>[5x]MSEKNVSIVVAASVLSSGIGINGQLPWSISEDLKFFSKITNNKCDSNKKNALIMG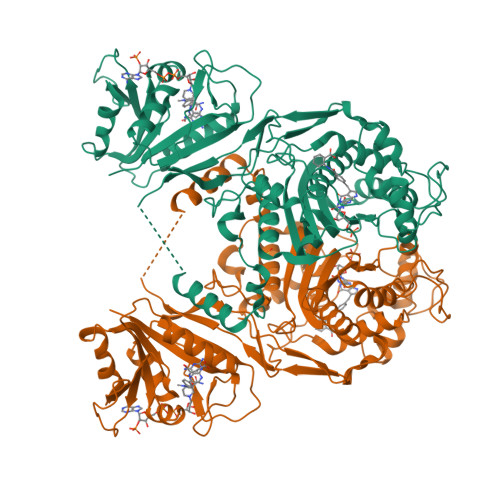RKTWDSIGRRPLKNRIIVVISSSLPQDEADPNVVVFRNLEDSIENLMNDDSIENIFVCGGESIYRDALKDNFVDRIYLTRVALEDIEFDTYFPEIPETFLPVYMSQTFCTKNISYDFMIFEKQEKKTLQNCDPARGQLKSIDDTVDLLGEIFGIRKMGNRHKFPKEEIYNTPSIRFGREHYEFQYLDLLSRVLENGAYRENRTGISTYSIFGQMMRFDMRESFPLLTTKKVAIRSIFEELIWFIKGDTNGNHLIEKKVYIWSGNGSKEYLERIGLGHREENDLGPIYGFQWRHYNGEYKTMHDDYTGVGVDQLAKLIETLKNNPKDRRHILTAWNPSALSQMALPPCHVLSQYYVTNDNCLSCNLYQRSCDLGLGSPFNIASYAILTMMLAQVCGYEPGELAIFIGDAHIYENHLTQLKEQLSRTPRPFPQLKFKRKVENIEDFKWEDIELIGYYPYPTIKMDMAV>[2x]MNDSNCFPFTKLSVQAQYERVQREFSLLLRQEDPRSISFATSLKNRHKNRYLDILANEATLYPQVTDAPGASTPYYINGNLIDLDLPHKFVACQAPVVQGIPDFLAMLYEKKISLVIM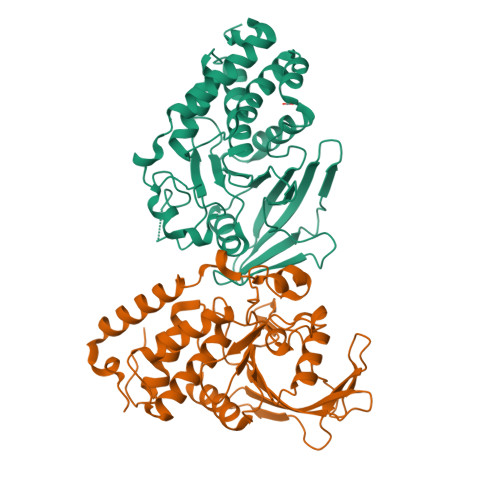VTKLEEGGFVKADRYWPEERGSGSIAVSGNCGLTISEDPGKAYEVEDELKITRRYLILQRADEPPHKFTQVQYTGWPDHGIPQSATSLEALLTNVKNSPTTVPVVVHCSAGIGRTGTLIGAYAALTHLERGTLTDTTVYDVVSAMRRQRFGMVQRMEQYFVIYLTLMCRLGVDIKALVGLLNSR> MTSMASLFSFTSPAVKRLLGWKQGDEEEKWAEKAVDALVKKLKKKKGAMEELEKALSSPGQPSKCVTIPRSLDGRLQVSHRKGLPHVIYCRVWRWPDLQSHHELKPLDICEFPFGSKQKEVCINPY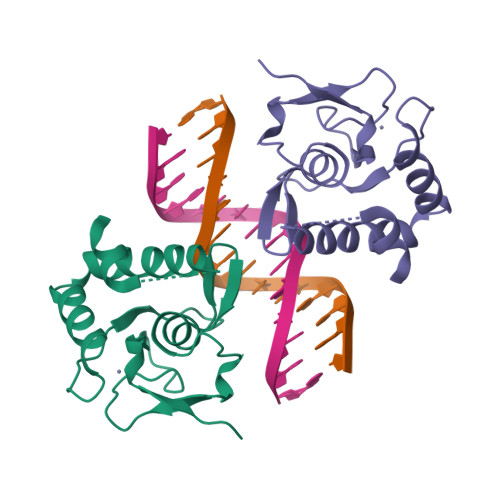HYKRVESPVLPPVLVPRLEHHHHH> MSIVRIAPEINLVMDTESGTVTQERKDSIQYSMEPVFERVDKL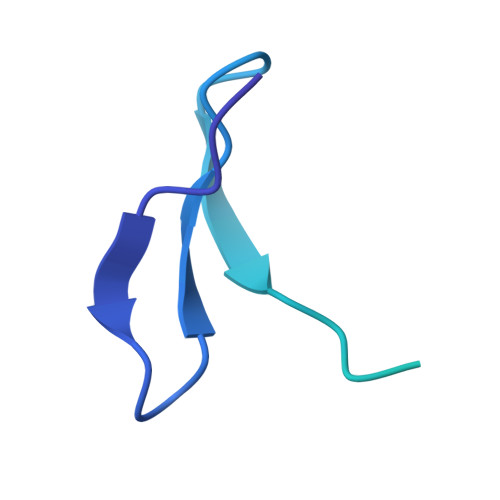DAIADDLVNSLSPSKPLLNTWPGRENTSYIAGIYSNSFYGIIVGLAFSGLLALIIYITRLMGGVV> QDDSRYTKFLTQHHDAKPKGRDDRYCERMMKRRSLTSPCKDVNTFIHGNKSNIKAICGANGSPYRENLRMSKSPFQVTTCKHTGGSPRPPCQYRASAGFRHVVIACEN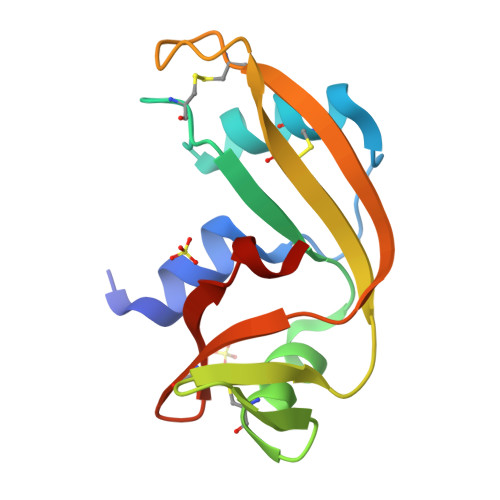GLPVHFDESFFSL> MEAEKKLFLKALKEKFEEDPKEKYTKFYTFGGWQQSARKREFVEANEKIVAEKRGGIPMYNPDIGVPLGQRKLMPYKLSGTDYIVEGDDLHFMNNAAIQQMWDDIRRTVIVGMDTGHAVLEKRLGVEVTPETINEYMATINHSLPGGAVVQEHMVEVHPSLAWDCYAKIFTGDDELADELDKKYLIDINKLFPEEQAEQLKAAIGKKTYQVSRVPTLVGRVCDGGTIARWSAMQIGMSFITAYKLCAGEAAIADFSYAAKHADVVGVGTALPARRSRGANEPGGIPFGVLCDIVQ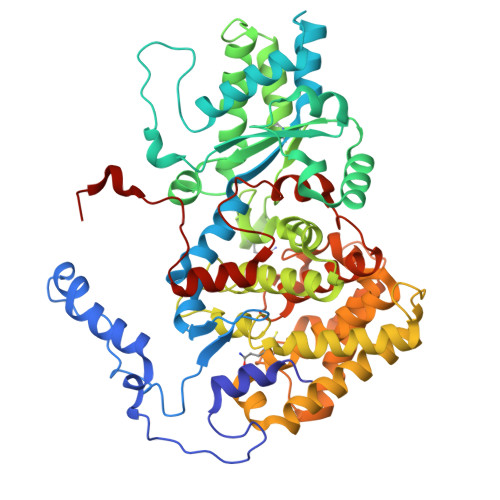TTRISDDPVEQSLEVVAVGAMLYDQVWLGSYMSGGVGFTQYATAAYTDDILDDFAYYGYEYVEKKYGINSTKPTMDVVEDIATEVTLYSLEQYDEFPTLLEDHFGGSQRAAVAAAASGISVCMATGNSNAGVNGWYLSQIMHKEYHSRLGFYGYDLQDQCGASNSLSIRNDEASPLELRGPNYPNYAMNVGHQGEYAGITQAAHSARKDAFAMNPLIKIAFADPSLVFDFARPRKECARGALREFEAAGERDVILPAK>[2x]KETAAAKFE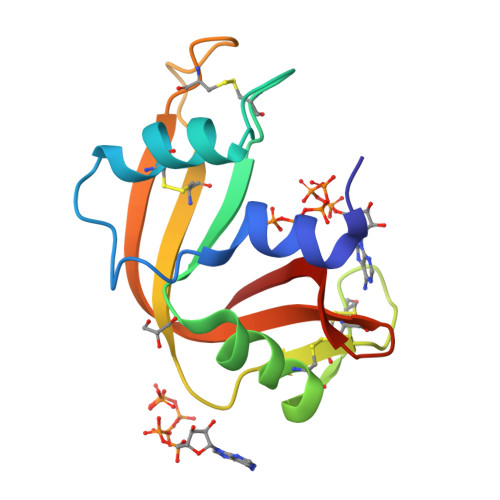RQHMDSSTSAASSSNYCNQMMKSRNLTKDRCKPVNTFVHESLADVQAVCSQKNVACKNGQTNCYQSYSTMSITDCRETGSSKYPNCAYKTTQANKHIIVACEGNPYVPVHFDASV>ANESAKDMTCQEFIDLNPKAMTPVAWWML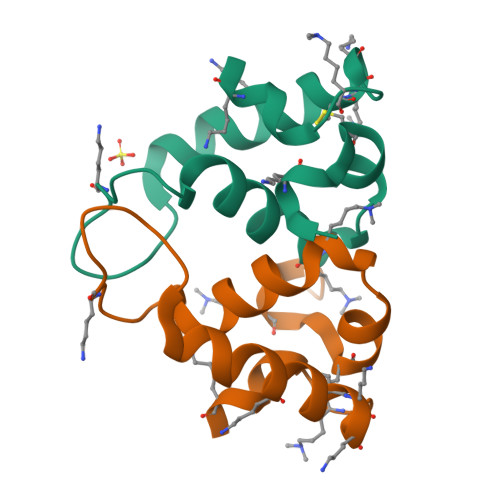HEETVYKGGDTVTLNETDLTQIPKVIEYCKKNPQKNLYTFKNQASNDLPN[4x]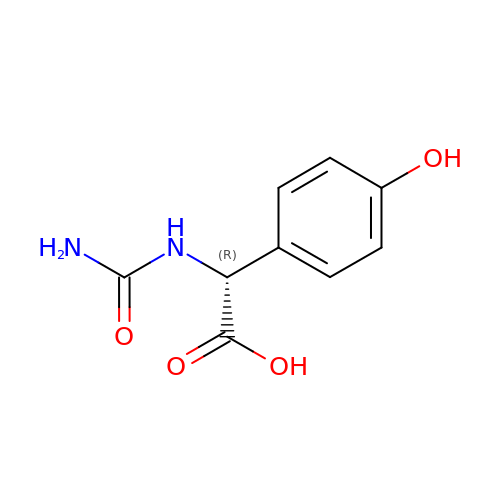(2~{R})-2-(aminocarbonylamino)-2-(4-hydroxyphenyl)ethanoic acid | C9 H10 N2 O4 | GSHIDXLOTQDUAV-SSDOTTSWSA-N> GSHTAEEDMEDDTSWRSEATFQFTVERFSRLSESVLSPPCFVRNLPWKIMVMPRFYPDRPHQKSVGFFLQCNAESDSTSWSCHAQAVLKIINYRDDEKSFSRRISHLFFHKENDWGFSNFMAWSEVTDPEKGFIDDDKVTFEVFVQADAPHGVAW;> E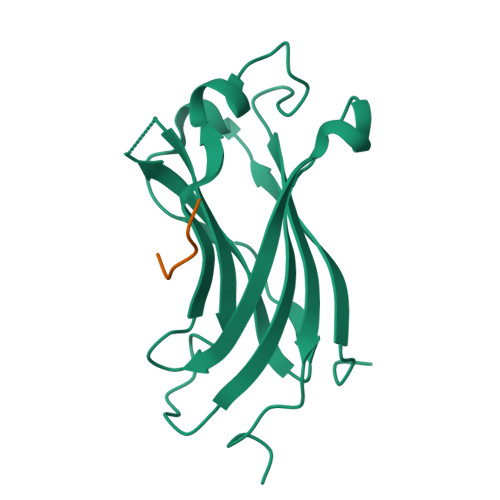KPSSS> GPMARTFILWLHGLGDSGPANEPIQTQFKSSELSNASWLFPSAPFNPVTCNNGAVMRSWFDVPEAPFKVGSPIDESSVLEAVKNVHAIIDQEIAEGTNPENVFICGLSQGGALTLASVLLYPKTLGGGAV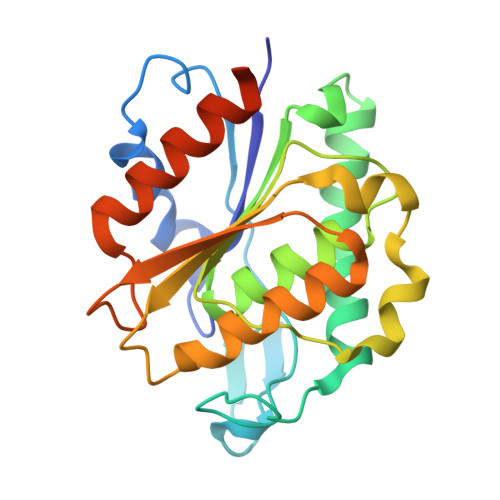LSGWVPFTSSIISQFPEEAKKTPILWSHGTDDRMVLFEAGQAALPFLKEAGVTCEFKAYPGLGHSISNKELKYIESWIKRRLKGSSSTCLQLNCLKEMFH> EGSPYVPVH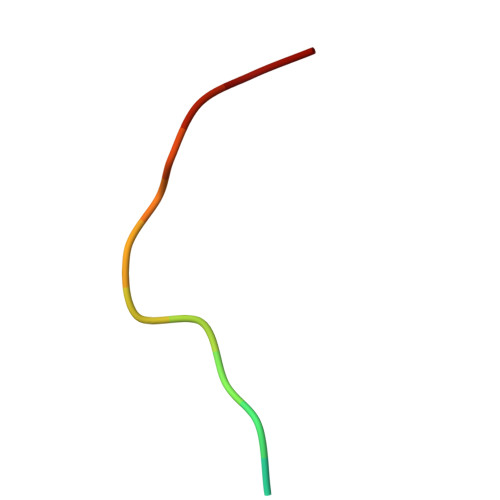YDASV>TYNGCSSSEQSALAAAASAAQSYVAESLSYLQTHTAATPRYTTWFGSYISSRHSTVLQHYTDMNSNDFSSYSFDCTCTAAGTFAYVYPNRFGTVYLCGAFWKAPTTGTDSQAGTLVHESSHFTRNGGTKDYAYGQAAAKSLATMDP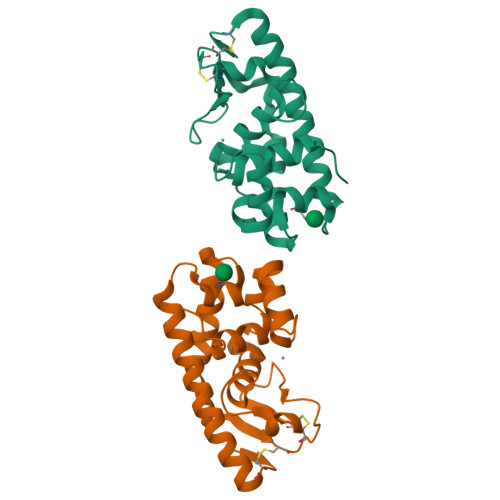DKAVMNADNHEYFSENNPAQS[2x]>[2x]XRMKQIEDKL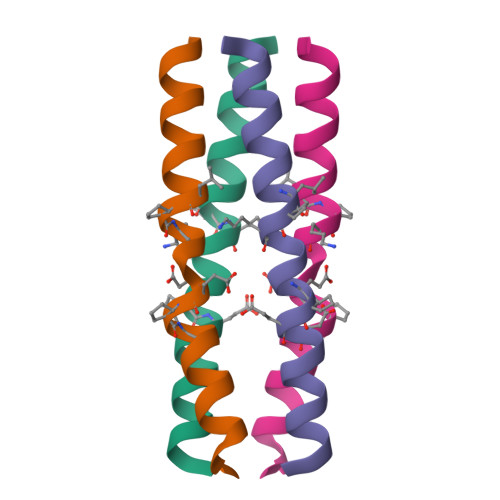EEILXKLXIEXELARIKKLLYER> MQLIDIGVNLTNSSFHDQQAAIVERALEAGVTQMLLTGTSLAVSEQALELCQQLDASGAHLFATAGVHPHDAKAWDTDSERQLRLLLSEPRVRAVGECGLDFNRDFSPRPLQEKALEAQLTLAAQLRLPVFLHERDASERLLAILKDYRDHLTGAVVHCFTGEREALFAYLDLDLHIGITGWICDERRGTHLHPLVGNIPEGRLMLESDAPYLLPRSLRPKPKSGRNEPAFLPEVLREVALHRGESAEHTAAHT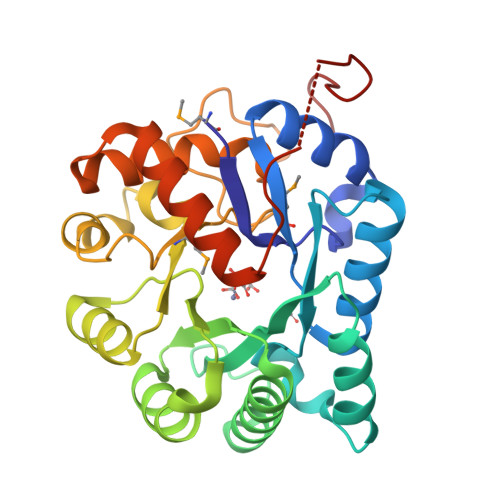TATARDFFQLPAENLYFQSHHHHHHWSHPQFEK>[2x]MDILLVD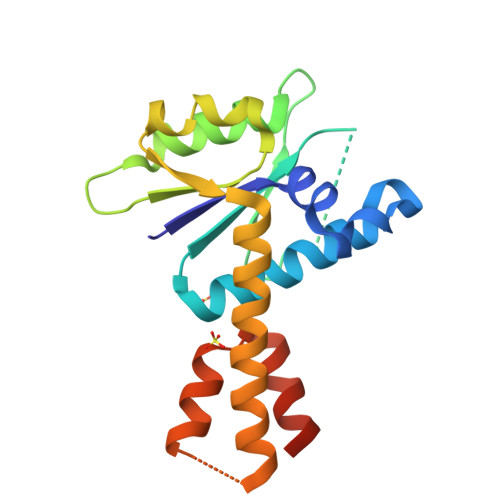GYNMIGAWPQLKDLKANSFEEARDVLIQKMAEYQSYTGNRVIVVFDAHLVKGLEKKQTNHRVEVIFTKENETADERIEKLAQALNNIATQIHVATSDYTEQWAIFGQGALRKSARELLREVETIERRIERRVRKITSEKPAGKIALSEEVLKTFEKLRRGDLDAAALEHHHHHH>GNGEYAWYYEGRNGWWQYDERTSRELEDAFSKGKKNTEMLIAGFLYVADLENMVQYRRNEHGRRRKIKRDIIDI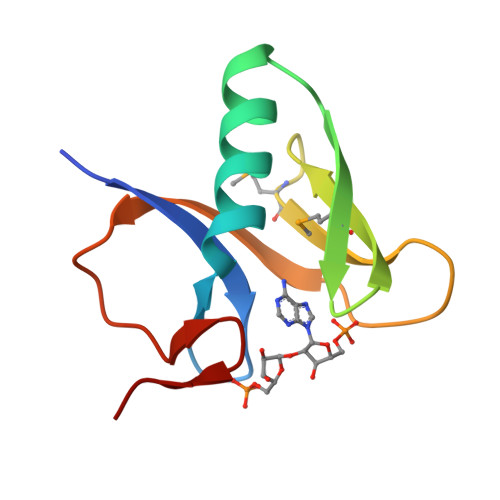PKKGVAGLRLD[2x]>GSRYQQPPVPYRQIDDCPAKARPQHIFYRRFLGKDGRRDPKCQWKFAVIFWGNDPYGLKKLSQAFQFGGVKAGPVSCLPHPGPDQSPITYCVYVYCQNKDTSKKVQMARLAWEASHPLAGNLQSSIVKFKKPLPLTQPG[10x]

The KSHV latency-associated nuclear antigen (kLANA) and the MHV68 mLANA (orf73) protein are required for latent viral replication and persistence. We solved the X-ray crystal structure of the C-terminal DNA binding domains (CTD) of kLANA and MHV-68 mLANA. The C-terminal domain (CTD) of LANA forms dimers, which bind two adjacent DNA sequences, the LANA binding sites (LBS1 & LBS2) in a single TR. Importantly, kLANA and mLANA CTD dimers undergo higher order oligomerization.

The structure of the kLANA fragment comprising residues 1013–1149 was solved by X-ray crystallography at a resolution of 2.60 Å, where electron density was observed for residues 1014–1147. kLANA(1013–1149) forms dimers that are stabilized by an eight-stranded antiparallel intermolecular β-barrel to which each monomer contributes four β-strands (β1–β4). The total dimer interface area is 2080 Å2 indicating that LANA is an obligate dimer. During our crystallization trials, we obtained three different crystal forms of the kLANA CTD, all of which contained higher order oligomers. The monoclinic and orthorhombic crystals of the kLANA CTD contained pentameric rings of dimers, whereas the cubic crystals contained tetrameric rings of dimers. In all structures the oligomerization interfaces are formed by helices α1 and α3, and the interface comprises an area of approx. 500 Å2. The angles between two neighboring LANA dimers range from 0° for mLANA, 72° for the kLANA pentameric rings to 90° for the kLANA tetrameric ring. Moreover, both pentameric ring structures of kLANA dimers display ring puckering, where the interface between two dimers is oriented out of the ring plane. DNA bending has been proposed to be a prerequisite for the initiation of DNA replication and a LBS1/2 containing probe was previously shown to be bent by ∼110° when both sites were occupied. Two adjacent kLANA dimers in our monoclinic crystals are perfectly oriented to bind and bend LBS1/2 to this extent. R1119 forms a positive charge at the bottom of a cleft, which is occupied by anions in the kLANA crystals.> GMDKSAKAPAITIFDHRGCSRAPKE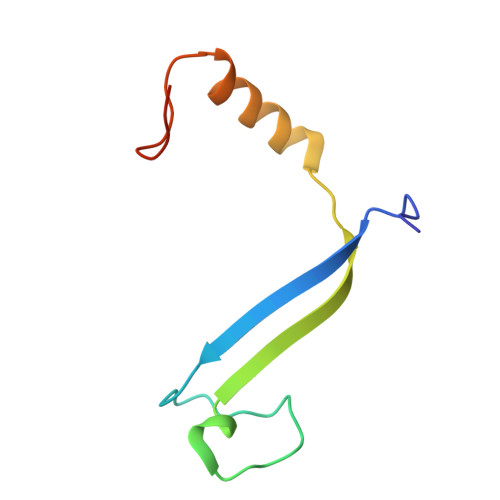SSAKSGSQDDEMLVKVASTKVTVSEDVAAKKLQEFIGFKEKGLDGSVIRKK>GC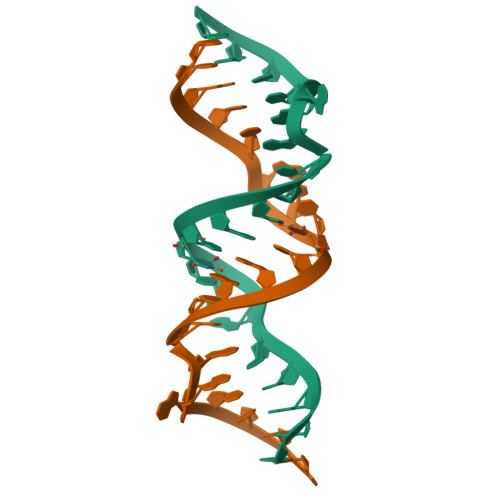GUCACCUCGAACAAGUCGC[4x]>SGMEELEQGLLMQPWAWLQLAENSLLAKVFITKQGYALLVSDLQQVWHEQVDTSVVSQRAKELNKRLTAPPAAFLCHLDNLLRPLLKDAAHPSEATFSCDCVADALILRVRSELSGLPFYWNFHCMLASPSLVSQHLIRPLMGMSLALQCQVRELATLLHMKDLEIQD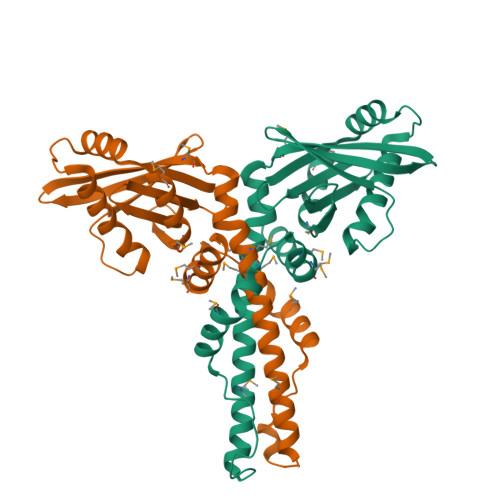YQESGATLIRDRLKTEPFEENSFLEQFMIEKLPEACSIGDGKPFVMNLQDLYMAVTTQEVQVGQKHQ[4x]> MATYKTPGVYIEEITKFPPSVAQVETAIPAFIGYTQFARTKPSVDSDDLILKPKRISSLLDFTTYYGGAQNEQGITVKLTDTLIEGAENRTINVPEPTFKSPYLMFYSLQMYFANGGGPCYIVSTGVYDDWSDSETPPTINFSDLESGLAVIRKEDEPTLLLFPDATNLPTDDEFYSLYNSALMQCNDLQDRFTILDTYSDQTYNDGVEDLDPIPALRNGINLTKD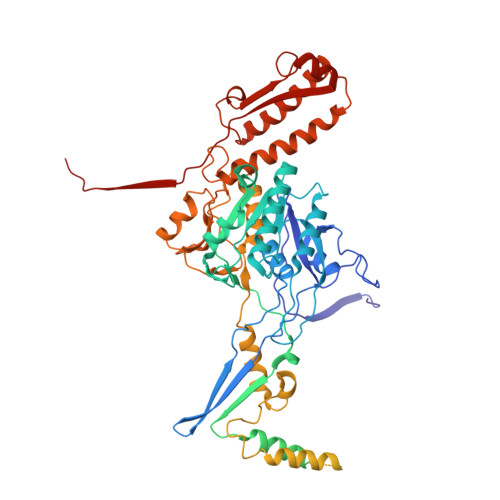YLKYGAAYYPFVQTILNYQYSADEIVIQHLSYNPNAIATALDNLNAVNGPTFIDAILDDLRDLSLPDISGEISDAVGFMYDDVDGFDIDGTFTTNSVKVANFASLVESVLSTLNELIDAKEEINKDVNSAIASSEEDNAIKTAISDALDVFNEDFEGADKIESVAKNLSDLLIKIKQADTNTKVENVLSINALNFSAEFEKLLTYDVNTGLTASVTLDLFANIGTRLDDIIAAVSAAEPIDVNNGKLNGRLLSDIEPLDNATYNTILLEINSHKVTLPPSSSMAGAYARVDNDRGVWKSPANIGLNYVSKPSVTVSHEEQESMNVHGTGKSVNAIRSFVGKGTLVWGARTLAGNDNEWRYISVRRFFNMAEESIKKATEQFVFEPNDGNTWVRVRAMIENFLILQWRAGALAGAKPEHAFYVKVGLGQTMTAQDILEGNMNVEIGLAVVRPAEFIILKFSHKMQES>[3x]MFDVIVVGGGPTGLMLAGELRLHGVRVLVLEKETEPTRQSRAQGLHVRSIEVMAQRGLLERFLERGH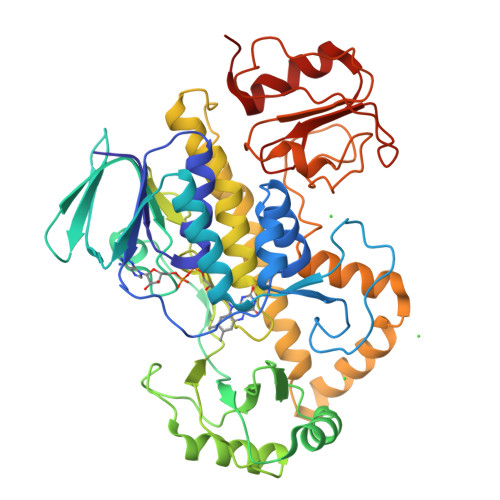TVAVGGFFAGLATSWPERLDTAHSYVLAVPQVITEQLLAEHATALGAEIRRGRALVGLRQDEDGVTVDLADGEQLRARYVVGCDGGRSTVRKLLGVAFPGEPSRVETLLGEMEMTASQEELTSVMTEVRKTQQRFGAMPLGDGVFRVVVPAEGVAEDRTASPTLDEFKQQLRAHAGTDFGVHSPRWLSRFGDATRQAERYRVDRVFLAGDAAHIHPPTGGQGLNLGIQDAFNLGWKLAAEVDGWAPEGLLDTYHAERHPVATEVLDNTRAQIQLMSTEPGPQAVRRLMAELVEFENVNRYLIEKITAISVRYDVGEGHELLGRRMRDLALKHGRLYERMHEGRGLLLDQTGRLSVAGWEDRVDHVVEVSEELDVPAVLLRPDGHVVWAGEDQQELLTRMPAWFGAATAG5'-PHOSPHOTHYMIDINE (3'-5')-PYROPHOSPHATE ADENOSINE 3'-PHOSPHATE | C20 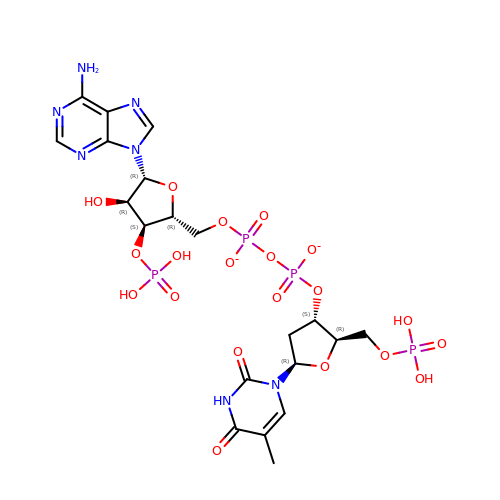H27 N7 O20 P4 | DQGQNMNTNSHMMC-SLFMBYJQSA-L> MENTENSVDSKSIKNLEPKIIHGSESMDSGISLDNSYKMDYPEMGLCIIINNKNFHKSTGMTSRSGTDVDAANLRETFRNLKYEVRNKNDLTREEIVELMRDVSK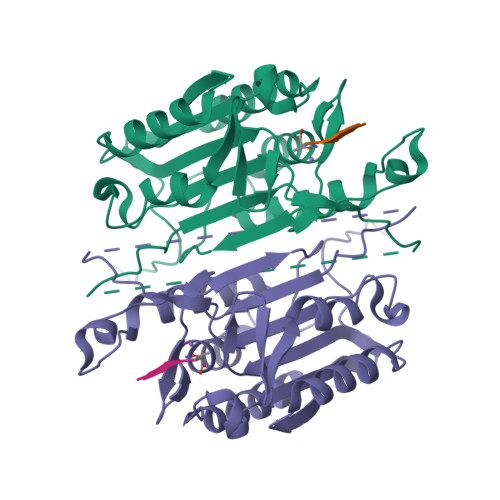EDHSKRSSFVCVLLSHGEEGIIFGTNGPVDLKKITNFFRGDRCRSLTGKPKLFIIQACRGTELDCGIETDSGVDDDMACHKIPVEADFLYAYSTAPGYYSWRNSKDGSWFIQSLCAMLKQYADKLEFMHILTRVNRKVATEFESFSFDATFHAKKQIPCIYSMLTKELYFYHL>MTQQITLIKDKILSDNYFTLHNITYDLTRKDGEVIRHKREVYDRGNGATILLYNTKKKTVVLIRQFRVATWVNGNESGQLIESCAGLLDNDEPEVCIRKEAIEETGYEVGEVRKLFELYMSPGGVTELIHFFIAEYSDNQRANAGGGVEDEA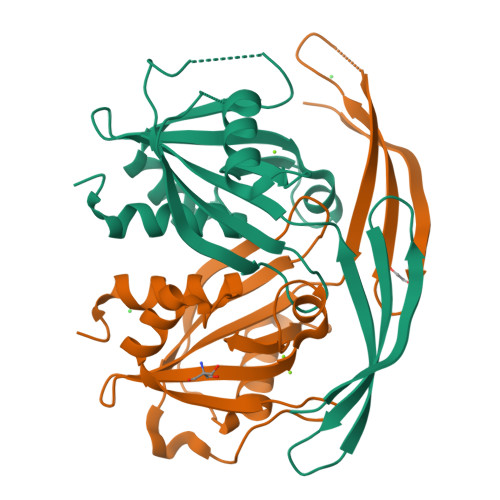IEVLELPFSQALEMIKTGEIRDGKTVLLLNYLQTSHLMD[2x]> GSHMASEKVAVETSVYLSELEWKSASTGYGEIQKDASCDGNTITLKGENGEKVSYDKGIGT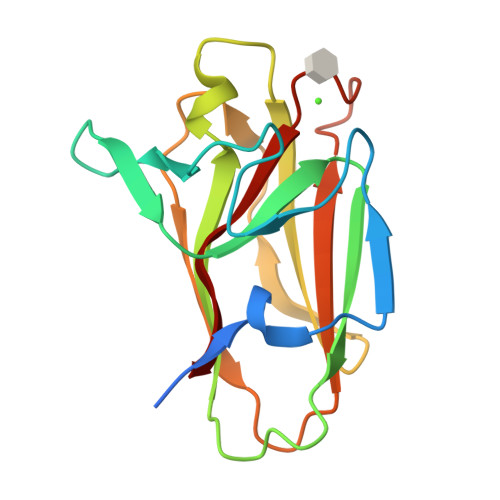HAHSEIVYSLEGLDYYDYFETFVGVDQEMAGTVASISFEVYLDNEKVFDSGLMTGDTTQKHVKVPIAGKNTLKLVVKDGGDSIGSDHGSFGDAKLT ATP citrate lyase (ACLY) is the predominant nucleocytosolic source of acetyl-CoA and is aberrantly regulated in many diseases making it an attractive therapeutic target. Structural studies of ACLY reveal a central homotetrameric core citrate synthase homology (CSH) module flanked by acyl-CoA synthetase homology (ASH) domains, with ATP and citrate binding the ASH domain and CoA binding the ASH-CSH interface to produce acetyl-CoA and oxaloacetate products. The specific catalytic role of the CSH module and an essential D1026A residue contained within it has been a matter of debate. Here, we report biochemical and structural analysis of an ACLY-D1026A mutant demonstrating that this mutant traps a (3S)-citryl-CoA intermediate in the ASH domain in a configuration that is incompatible with the formation of acetyl-CoA, is able to convert acetyl-CoA and OAA to (3S)-citryl-CoA in the ASH domain, and can load CoA and unload acetyl-CoA in the CSH module.

An ACLY-D1026A—substrates complex refined without symmetry (ACLY-D1026A—substrates-asym) reveals three symmetric and one asymmetric conformation. The symmetric ASH domains reveal an ASH active site and corresponding CSH domain containing bound (3S)-citryl-CoA and non-canonical CoA, respectively, as in the symmetric structure. Multiple rounds of 3D hetero refinement classification on the asymmetric particles (ACLY-D1026A—substrates-asym-int and ACLY-D1026A-substartes-asym in Table 1) revealed a large amount of conformational flexibility within this domain. The asymmetric ASH domain did not contain traceable cryo-EM density for a bound ligand, but instead, the CSH domain did contain cryo-EM density that could be tentatively modeled as CoA +  citrate, although (3 S)-citryl-CoA could also be modeled. A superposition of the ASH-bound (3 S)-citryl-CoA/CSH-bound non-productive CoA pair with the CSH-bound non-canonical CoA reveals the mutually exclusive nature of these two binding states. The relative positions of these ligands is consistent with CoA bound to the CSH in a pre-translocated loaded position, which moves to the ASH for the formation of the (3S)-citryl-CoA intermediate, and that bound non-canonical CoA serving to trap (3 S)-citryl-CoA within the ASH domain. If the ligand bound to the CSH domain is (3 S)-citryl-CoA, this could represent an “unloaded” (3 S)-citryl-CoA, which could not form acetyl-CoA and OAA products in the ASH. In either case, this asymmetric structure is consistent with the allosteric regulation of the ASH domain for ACLY catalysis.

>[4x]MSAKAISEQTGKELLYKFICTTSAIQNRFKYARVTPDTDWARLLQDHPWLLSQNLVVKPDQLIKRRGKLGLVGVNLTLDGVKSWLKPRLGQEATVGKATGFLKNFLIEPFVPHSQAEEFYVCIYATREGDYVLFHHEGGVDVGDVDAKAQKLLVGVDEKLNPEDIKKHLLVHAPEDKKEILASFISGLFNFYEDLYFTYLEINPLVVTKDGVYVLDLAAKVDATADYICKVKWGDIEFPPPFGREAYPEEAYIADLDAKSGASLKLTLLNPKGRIWTMVAGGGASVVYSDTICDLGGVNELANYGEYSGAPSEQQTYDYAKTILSLMTREKHPDGKILIIGGSIANFTNVAATFKGIVRAIRDYQGPLKEHEVTIFVRRGGPNYQEGLRVMGEVGKTTGIPIHVFGTETHMTAIVGMALGHRPIPNQPPTAAHTANFLLNASGSTSTPAPSRTASFSESRADEVAPAKKAKPAMPQDSVPSPRSLQGKSTTLFSRHTKAIVWGMQTRAVQGMLDFDYVCSRDEPSVAAMVYPFTGDHKQKFYWGHKEILIPVFKNMADAMRKHPEVDVLINFASLRSAYDSTMETMNYAQIRTIAIIAEGIPEALTRKLIKKADQKGVTIIGPATVGGIKPGCFKIGNTGGMLDNILASKLYRPGSVAYVSRSGGMSNELNNIISRTTDGVYEGVAIGGDRYPGSTFMDHVLRYQDTPGVKMIVVLGEIGGTEEYKICRGIKEGRLTKPIVCWCIGTCATMFSSEVQFGHAGACANQASETAVAKNQALKEAGVFVPRSFDELGEIIQSVYEDLVANGVIVPAQEVPPPTVPMDYSWARELGLIRKPASFMTSICDERGQELIYAGMPITEVFKEEMGIGGVLGLLWFQKRLPKYSCQFIEMCLMVTADHGPAVSGAHNTIICARAGKDLVSSLTSGLLTIGDRFGGALDAAAKMFSKAFDSGIIPMEFVNKMKKEGKLIMGIGHRVKSINNPDMRVQILKDYVRQHFPATPLLDYALEVEKITTSKKPNLILNVAGLIGVAFVDMLRNCGSFTREEADEYIDIGALNGIFVLGRSMGFIGHYLDQKRLKQGLYRHPWDDISYVLPEHMSM> APDSVDYRKKGYVTP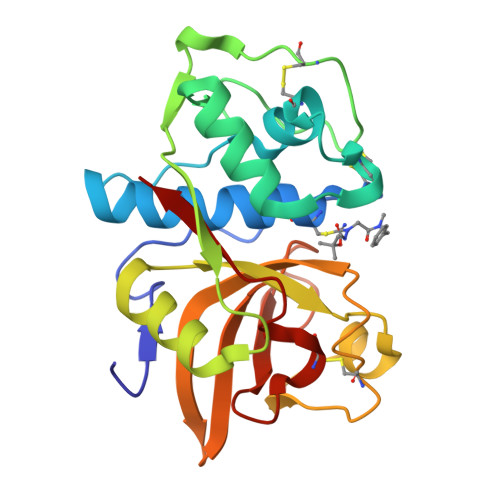VKNQGQCGSCWAFSSVGALEGQLKKKTGKLLNLSPQNLVDCVSENDGCGGGYMTNAFQYVQKNRGIDSEDAYPYVGQEESCMYNPTGKAAKCRGYREIPEGNEKALKRAVARVGPVSVAIDASLTSFQFYSKGVYYDESCNSDNLNHAVLAVGYGIQKGNKHWIIKNSWGENWGNKGYILMARNKNNACGIANLASFPKM>DGVDIY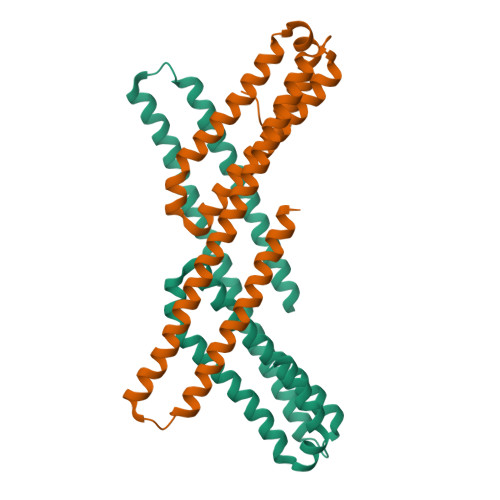FGMPGEISEHEGFLRAKMDLEERRMRQINEVMREWAMADNQSKNLPKADRQALNEHFQSILQTLEEQVSGERQRLVETHATRVIALINDQRRAALEGFLAALQADPPQAERVLLALRRYLRAEQKEQRHTLRHYQHVAAVDPEKAQQMRFQVHTHLQVIEERVNQSLGLLDQNPHLAQELRPQIQELLHSEHLGPSE[2x]CEPHALOTHIN | C16 H16 N2 O6 S2 | 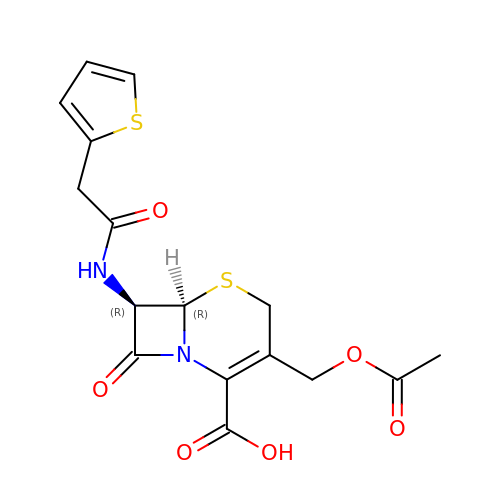XIURVHNZVLADCM-IUODEOHRSA-N>MLPRPSGTYAGLPIADYGDAPPLSTKTMFWRTSPEKLPPGAWEPAYLGSKDERVDGPSLQQVMRDQLKPYSEPRGLLPPQEILDAVCDAIENRLENTLEPQKPWTFKKACESLDKNTSSGYPYHKQKSKDWTGSAFIGDLGDQATHANNMYEMGKSMRPIYTAALKDELVKPDKIYGKIKKRLLWGSDLGTMIRAARAFGPFCDALKETCIFNPIRVGMSMNEDGPFIFARHANFRYHMDADYTRWDSTQQRAILKR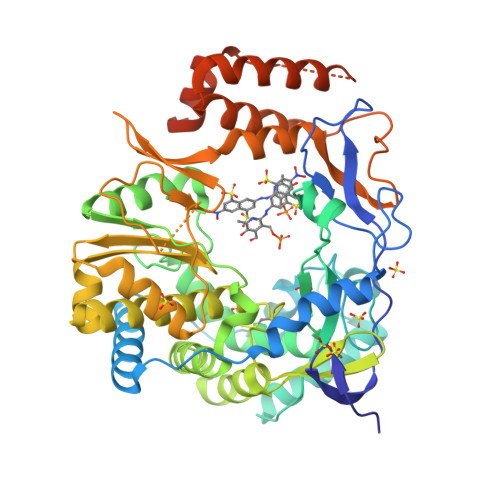AGDIMVRLSPEPDLARVVMDDLLAPSLLDVGDYKIVVEEGLPSGCPCTTQLNSLAHWILTLCAMVEVTRVDPDIVMQESEFSFYGDDEVVSTNLELDMVKYTMALRRYGLLPTRADKEEGPLERRQTLQGISFLRRAIVGDQFGWYGRLDRASIDRQLLWTKGPNHQNPFETLPGHAQRPSQLMALLGEAAMHGEKYYRTVASRVSKEAAQSGIEMVVPRHRSVLRWVRFGTMDAETPQERSAVFVNEDELEHHHHHH[3x]>NKSLVDQMLVELDKKISAQMDEILHNSQFQAMESAWRGLKLFVDRTDFRENNKVEILHVTKDELLEDFEFAPETAQSGLYKHVYSAGYGQFGGEPVGAIIGNYAFTPSTPDMKLLQYMGALGAMAHAPFISSVGPEFFGIDSFEELPNIKDLKSTFESPKYTKWRSLRESEDARYLGLTAPRFLLRVPYDPIENPVKSFNYAENVSASHEHYLWGNTAFAFA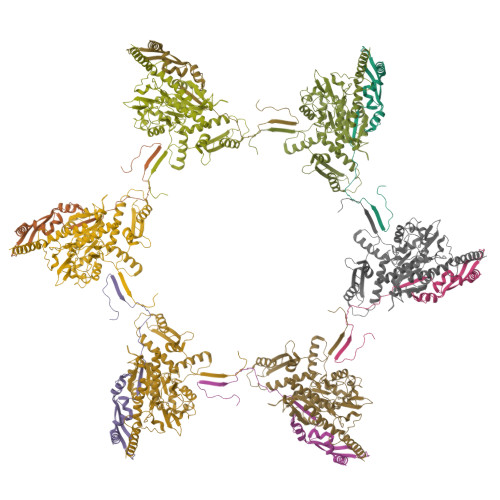TRLTDSFAKYRWCPNIIGPQSGGAVEDLPVHVFESMGALQSKIPTEVLITDRKEFELAEEGFIALTMRKGSDNAAFFSANSIQKPKVFPNTKEGKEAETNYKLGTQLPYMMIINRLAHYVKVLQREQIGAWKERQDLERELNSWIKQYVADQENPPADVRSRRPLRAARIEVMDVEGNPGWYQVSLSVRPHFKYMGANFELSLVGRLD[6x];>SKEGSVAPKERINIKYIPATGDAQAEAEVELPLKTLVVGDFKGHAEQTPLEERATVTVDKNNFEAVMRESELKITATVKNKLTDDENAELPVELNFKSLADFAPDAVASQVPELKKLIELREALVAL[6x]>[4x]MAFELPNLPYGFRALEPHIDQQTMEIHHDKHHNTYVTKLNAAVEGTDLESKSIEEIVANLDSVPENIQTAVRNNGGGHLNHSLFWELLTPNSEEKGTVVDKIKEQWGSLDAFKEEFA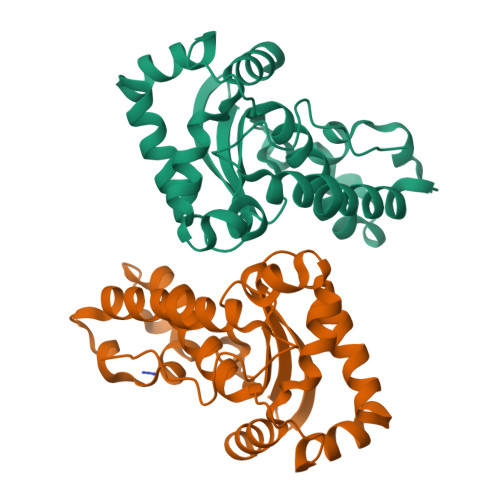NQAAARFGSGWAWLVVNDGKLEIVTTPNQDNPLTEGKTPILGLDVWEHAYYWKYQNKRPDYISAFWNVVNWEKVDELYNAAKHHHHHH> MANRATSAFLDNPHPVGVNYVDEGSRQFVAVAELLASKLIDSSRESDESNSDVPFVQAYSKFADDNPRHLRVKTGGKMANALTNVIRSYYSINAPAIVPQVEIDRLASKATVSGDMYNSYAIFNSVPIVEVLSPARTTVSIVGSDRADVTMLNTGAGAANITFNFGQIAETVILKGSVPFQLARLNQPMPAARFTYKLRPLDGPFIVVLPVGNPLVISATAATRIQVPLAFNKALVESGFQTAMNDGLFDIQNVNYYSSFDEFIISQYHAQDGINRVSTCVILGLALQA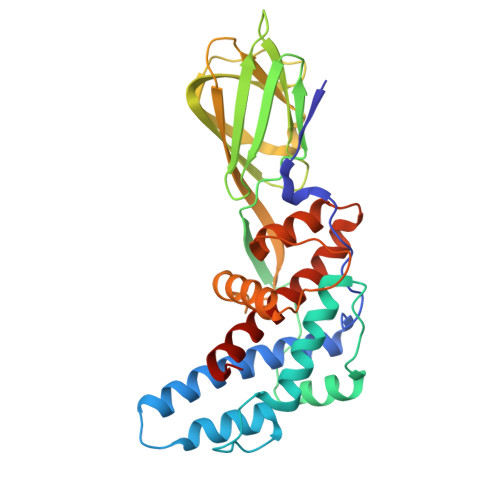YDQMRRALPVRRV>[2x]MRALTLKDILNGTFSYKTFFPNWISGQEYLHQSADNNIVLYNIETGQSYTILSNRTMKSVNASNYGLSPDRQFVYLESDYSKLWRYSYTATYYIYDLSNGEFVRGNELPRPIQYLCWSPVGSKLAYVYQNNIYLKQRPGDPPFQITFNGRENKIFNGIPDWVYEEEMLATKYALWWSPNGKFLAYAEFNDTDIPVIAYSYYGDEQYPRTINIPYPKAGAKNPVVRIFIIDTTYPAYVGPQEVPVPAMIASSDYYFSWLTWVTDERVCLQWLKRVQNVSVLSICDFREDWQTWDCPKTQEHIEESRTGWAGGFFVSTPVFSYDAISYYKIFSDKDGYKHIHYIKDTVENAIQITSGKWEAINIFRVTQDSLFYSSNEFEEYPGRRNIYRISIGSYPPSKKCVTCHLRKERCQYYTASFSDYAKYYALVCYGPGIPISTLHDGRTDQEIKILEENKELENALKNIQLPKEEIKKLEVDEITLWYKMILPPQFDRSKKYPLLIQVYGG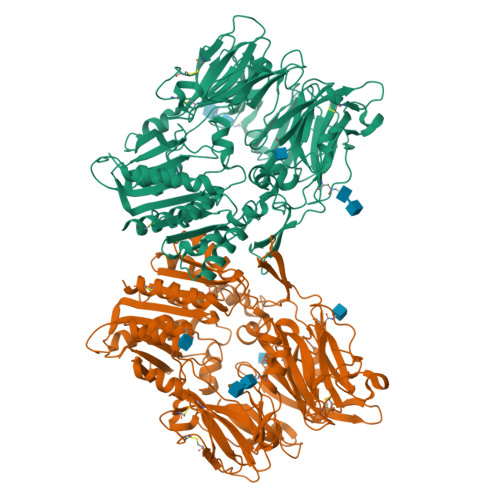PCSQSVRSVFAVNWISYLASKEGMVIALVDGRGTAFQGDKLLYAVYRKLGVYEVEDQITAVRKFIEMGFIDEKRIAIWGWSYGGYVSSLALASGTGLFKCGIAVAPVSSWEYYASVYTERFMGLPTKDDNLEHYKNSTVMARAEYFRNVDYLLIHGTADDNVHFQNSAQIAKALVNAQVDFQAMWYSDQNHGLSGLSTNHLYTHMTHFLKQCFS>GSMDQRQKLQHWIHSCLRKADKNKDNKMNFKELKDFLKELNIQVDDGYARKIFRECDHSQTDSLEDEEIETFYKMLTQRAEIDRAFEEAAGSAETLSVERLVTFLQHQQREEEAGPALALSLIERYEPSETAKAQRQMTKDGFLMYLLSADGNAFSLAHRRVYQDMDQPLSHYLVSSSHNTYLLEDQLTGPSSTEAYIRALCKGCRCLELDCWDGPNQEPIIYHGYTFTSKILFCDVLRAIRDYAFKASPYPVILSLENHCSLEQQRVMARHLRAILGPILLDQPLDGVTTSLPSPEQLKGKILLKGKKLGGLLPAGGENGSEATDVSDE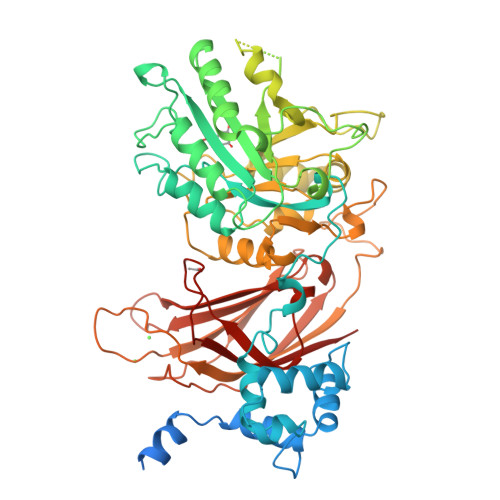VEAAEMEDEAVRSQVQHKPKEDKLKLVPELSDMIIYCKSVHFGGFSSPGTSGQAFYEMASFSESRALRLLQESGNGFVRHNVSCLSRIYPAGWRTDSSNYSPVEMWNGGCQIVALNFQTPGPEMDVYLGCFQDNGGCGYVLKPAFLRDPNTTFNSRALTQGPWWRPERLRVRIISGQQLPKVNKNKNSIVDPKVIVEIHGVGRDTGSRQTAVITNNGFNPRWDMEFEFEVTVPDLALVRFMVEDYDSSSKNDFIGQSTIPWNSLKQGYRHVHLLSKNGDQHPSATLFVKISIQD[2x]>[4x]MGTKKSAAEASKKPRQKRTATKAYNVTQAFGRRGPE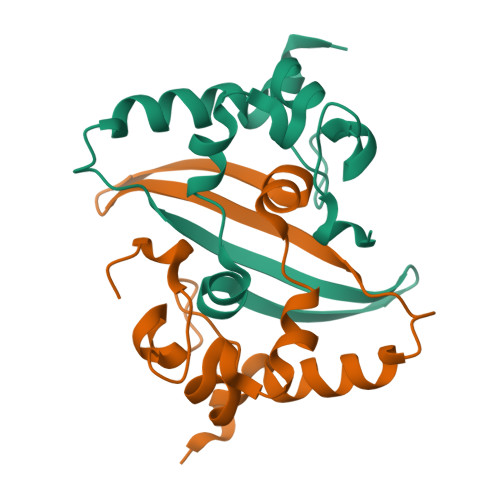QTQGNFGDQELIRQGTDYKHWPQIAQFAPSASAFFGMSRIGMEVTPSGTWLTYTGAIKLDDKDPNFKDQVILLNKHIDAYKTFP>MKGQETRGFQSEVKQLLHLMIHSLYSNKEIFLRELISNASDAADKLRFRALSNPDLYEGDGELRVRVSFDKDKRTLTISDNGVGMTRDEVIDHLGTIAKSGTKSFLESLGSDQAKDSQLIGQFGVGFYSAFIVADKVTVRTRAAGEKPENGVFWESAG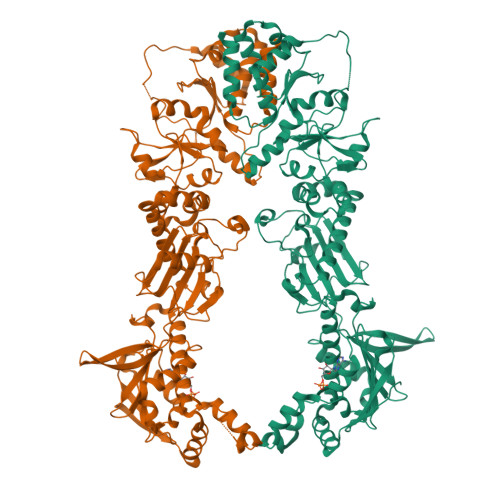EGEYTVADITKEDRGTEITLHLREGEDEFLDDWRVRSIISKYSDHIALPVEIEKREEKDGETVISWEKINKAQALWTRNKSEITDEEYKEFYKHIAHDFNDPLTWSHNRVEGKQEYTSLLYIPSQAPWDMWNRDHKHGLKLYVQRVFIMDDAEQFMPNYLRFVRGLIDSSDLPLNVSREILQDSTVTRNLRNALTKRVLQMLEKLAKDDAEKYQTFWQQFGLVLKEGPAEDFANQEAIAKLLRFASTHTDSSAQTVSLEDYVSRMKEGQEKIYYITADSYAAAKSSPHLELLRKKGIEVLLLSDRIDEWMMNYLTEFDGKPFQSVSKVDESLEKLADEVDESAKEAEKALTPFIDRVKALLGERVKDVRLTHRLTDTPAIVSTDADEMSTQMAKLFAAAGQKVPEVKYIFELNPDHVLVKRAADTEDEAKFSEWVELLLDQALLAERGTLEDPNLFIRRMNQLLVS[4x]>MVTPEGNVSLVDESLLVGVTDEDRAVRSAHQFYERLIGLWAPAVMEAAHELGVFAALAEAPADSGELARRLDCDARAMRVLLDALYAYDVIDRIHDTNGFRYLLSAEARECLLPGTLFSLVGKFMHDINVAWPAWRNLAEVVRHGARDTSGAESPNGIAQEDYESLVGGINFWAPPIVTTLSRKLRASGRSGDATASVLDVGCGTGLYSQLLLREFPRWTATGLDVERIATLANAQALRLGVEERFATRAGDFWRGGWGTGYDLVLFANIFHLQTPASAVRLMRHAAACLAPDGLVAVVDQIVDADREPKTPQDRFALLFAASMTNTGGGDAYTFQEYEEWFTAAGLQRIETLDTPMHRILLA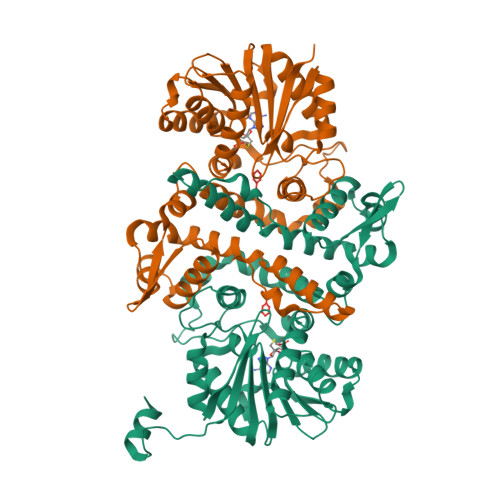RRATEPSAVPEGQASENLYFQ[2x]> GPGSEFELPLPEGWEEARDFDGKVYYIDHRNRTTSWIDPRDRYTKPLTFADCISDELPLGWEEAYDPQVGDYFIDHNTKTTQIEDPRVQWRREQEHMLKDYLVVAQEALSAQKEIYQVKQQRLELAQQEYQQLH;> GPGSRPK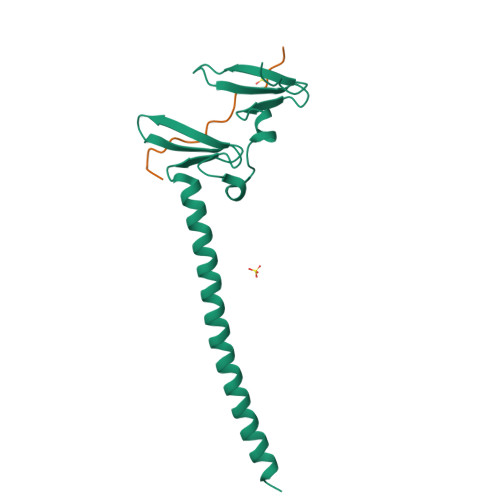NMTPYRSPPPYVPP>EEEGRIRAMRAARSLGERTVTELILQHQNPQQLSSNLWAAVRARGCQFLGPAMQEEALKLVLLALEDGSALSRKVLVLFVVQRLEPRFPQASKTSIGHVVQLLYRASCFKVTKRDEDSSLMQLKEEFRTYEALRREHDSQIV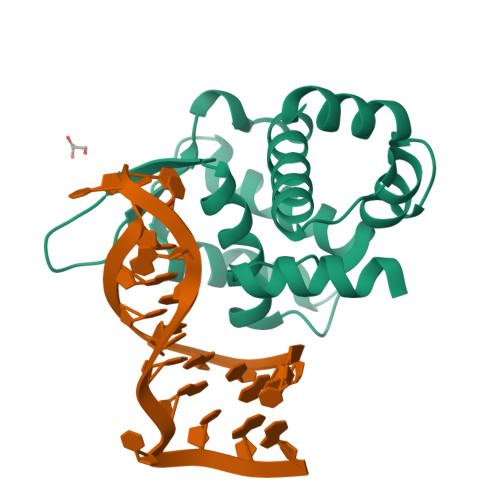QIAMEAGLRIAPDQWSSLLYGDQSHKSHMQSIIDKLQT[2x]N-[2-(5,8-dimethoxy-2-oxo-1,2-dihydroquinolin-3-yl)ethyl]-2-iodobenzamide | C20 H19 I N2 O4 | 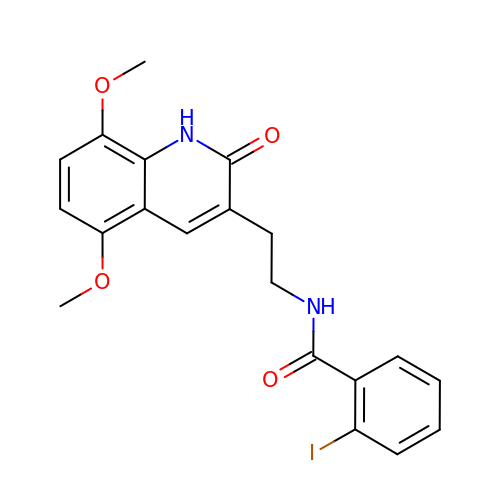RJARQBKOBDUFBP-UHFFFAOYSA-N>GGELMIKSSNAFDVIELSSQIQRYASLSKINNRTNPILKDNKAKEFKDADLKWLKLENCPTAGDVPTTGNNNDLQDQFIACDADYRKGDLSYFGSQFEFSTYVHPSNPEIQRQIKQVVSYFQYRGMERAFIGDAAGYVISEAKKKGFSAQDYRIVLIEPDRVGYFESNAISYEEFIENPSARENFLLKATKDRTLALAVSLAQTGEIAMQRDGSVAFLEDSELCWDTAAGSAKSCLSVRYDTVGNKTELDLKQIDVVSAKGLSFESDGKTKTPVVSTYETFQDGGRAKTINAIECPTGLNNRFAAVVSSFSTAGQNANFSSESAKDSQGTTQKDGSKGPHALLSGISLNWTLTNKVWDVTASIGIESGILPTSGIDSGSLLRNPKSLSFIAFQWCEN[3x]

The toxin-coregulated pilus (TCP), an operon-encoded type IVb pilus (T4bP), plays a crucial role in this process, which requires an additional secreted protein, TcpF, encoded on the same TCP operon; however, its mechanisms of secretion and function remain elusive. Here, we demonstrated that TcpF interacts with the minor pilin, TcpB, of TCP and elucidated the crystal structures of TcpB alone and in complex with TcpF. Repetitive TcpA units form the filament structure, whereas TcpB displays multiple functions, such as efficient pilus assembly, pilus retraction, and CTXφ uptake. The structural analyses reveal how TCP recognizes TcpF and its secretory mechanism via TcpB-dependent pilus elongation and retraction.

TcpB comprises three domains, of which the crystal structures of C-terminal domains (domain 2 and domain 3) were recently resolved, showing that these two domains consist of β-strand–rich folds forming a homotrimeric pilus initiation complex. The structure of TcpB domain 1 remains unknown and is predicted to be a pilin-like domain based on the similarity of its sequence with other T4b pilins. We then analyzed the structure of TcpB alone and in complex with the TcpF (1–15) peptide. The structure of TcpB domain 1 adopts an α/β-roll fold similar to that of other type IV pilins, but the α/β loop connecting the α1 helix to the central β-sheet is outstandingly different. The α/β loop of TcpB consists of 64 residues, which are remarkably longer than the 38 residues of major pilin TcpA, and has a disulfide bond formed between Cys85 and Cys107 in the loop. This disulfide bond in the α/β loop can also be observed in domain 1 of ETEC minor pilin CofB and likely stabilizes the longer α/β loops of these minor pilins. In general, type IV pilins form a disulfide bond in the D-region; however, TcpB has a disulfide bond between Cys85 and Cys107 in the α/β loop instead of the D-region. To confirm the association of TcpB and TcpF in solution, we performed sedimentation velocity-analytical ultracentrifugation. This experiment demonstrated that TcpB (43.5 kDa) is a trimer with an estimated molecular mass of 120.0 kDa. The crystal structure of TcpB domain 1 that was determined here allows us to simulate this situation by replacing one TcpA molecule at the bottom of the TCP filament model with one TcpB subunit. In this model, Glu5 of TcpB can interact with the Met1 amine of TcpA.octacosan-1-ol | C28 H58 O | 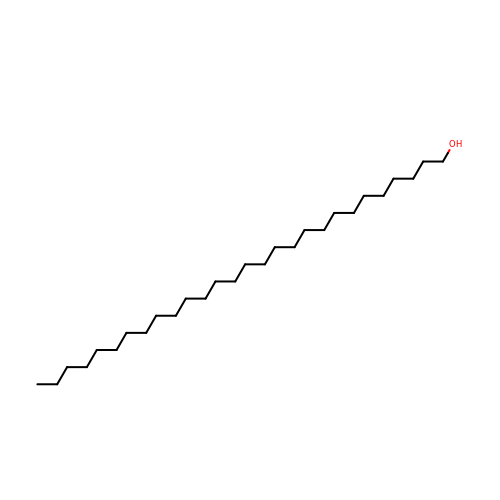CNNRPFQICPFDPO-UHFFFAOYSA-N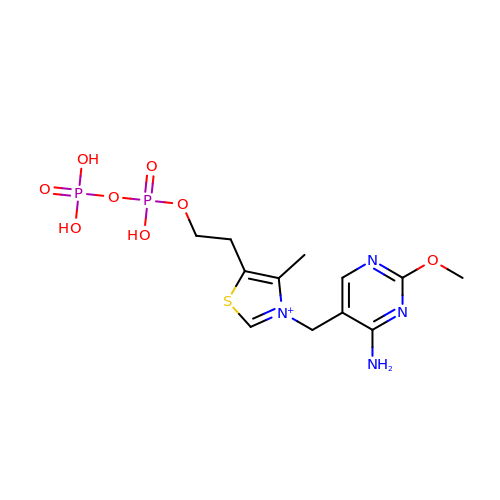2-[3-[(4-azanyl-2-methoxy-pyrimidin-5-yl)methyl]-4-methyl-1,3-thiazol-5-yl]ethyl phosphono hydrogen phosphate | C12 H19 N4 O8 P2 S | PWBCVHDHRGCQHM-UHFFFAOYSA-O> ITAVETRTIVRF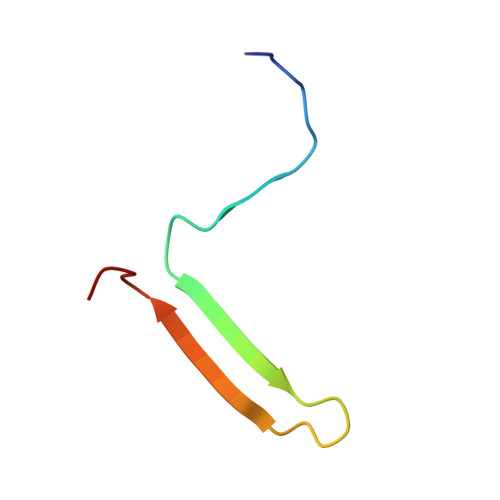NRPFLMIIVDHFTWSIFFMSKVTNPKQA>MEAVPRMPMIWLDLKEAGDFHFQPAVKKFVLKNYGENPEAYNEELKKLELLRQNAVRVPRDFEGCSVLRKYLGQLHYLQSRVPMGSGQEAAVPVTWTEIFSGKSVAHEDIKYEQACILYNLGALHSMLGAMDKRVSEEGMKVSCTHFQCAAGAFAYLREHFPQAYSVDMSRQILTLNVNLMLGQAQECLLEKSMLDNRKSFLVARISAQVVDYYKEACRALENPDTASLLGRIQKDWKKLVQMKIYYFAAVAHLHMGKQAEEQQKFGERVAYFQSALDKLNEAIKLAKGQPDTVQDALRFTMDVIGGKYNSAKKDNDFIYHEAVPALDTLQPVKGAPLVKPLPVNPTDPAVTGPDIFAKLV[2x];> KKKEEEDDDMKELENWAGSM

His domain protein tyrosine phosphatase (HD-PTP/PTPN23) is a tumor suppressor that regulates mitogenic receptor downregulation, endocytic recycling, and cell migration (Chen et al., 2012, Doyotte et al., 2008, Kharitidi et al., 2015, Lee et al., 2007, Ma et al., 2015, Manteghi et al., 2016). A central feature of HD-PTP function is the ability of its Bro1 domain to recruit CHMP4, the major subunit of the ESCRT-III membrane remodeling protein complex (Doyotte et al., 2008, Ichioka et al., 2007, Parkinson et al., 2015). Crystallographic structures of the HD-PTPBro1 domain in complex with the relevant binding regions of SARA, endofin, and all three human CHMP4 isoforms reveal that SARA and endofin binding is similar to that of CHMP4 at the conserved site, but critically extends into a neighboring specific pocket unique to HD-PTP. Altogether, this study identifies the Bro1 domain of HD-PTP as a highly selective interaction hub that coordinates recruitment of endosomal signaling adaptors versus MVB sorting and receptor degradation.

Y2H experiments confirmed that this region is also relevant for binding to HD-PTP, since CHMP4B lacking the C-terminal six amino acids (C4BΔCT) did not bind AlixBro1-V or HD-PTPBro1-CC, while full-length CHMP4B did. CoIP confirmed that CHMP4B-FL, but not C4BΔCT, binds to HD-PTPBro1-CC. Next, peptides designed from the C-terminal 18–20 residues of CHMP4A, CHMP4B, and CHMP4C were evaluated for binding to HD-PTPBro1. Interestingly, CHMP4 peptides showed much lower affinity to HD-PTPBro1 compared with the SARA/endofin peptides, with KD values of 132 ± 7 μM for CHMP4A, 85 ± 2 μM for CHMP4B, and 89 ± 1 μM for CHMP4C. For the CHMP4 peptides only 11 residues are clearly visible in the electron density maps, whereas 20 residues are visible for the SARA and endofin peptides. All three CHMP4 peptides bind in the same way across helices H5, H6, and H7 of HD-PTPBro1, and form similar van der Waals contacts with a number of conserved residues, including the critical L202/I206 pair. Additional contacts occur with hydrophobic residues at the proline-rich C-terminal region of HD-PTPBro1 (see Table 2 for a list of all interactions). The main CHMP4 anchoring residues are a Leu and a Trp present in all three isoforms (L217 and W220 in CHMP4A and CHMP4B, L228/W231 in CHMP4C), which contact HD-PTPBro1 residues L189, L202, and I206 from two hydrophobic pockets between H5 and H6 and H6 and H7. Thus, binding of CHMP4A/B/C to HD-PTPBro1 requires rearrangement of these side chains to accommodate the critical CHMP4 Leu and Trp residues. Binding of full-length CHMP4B to HD-PTPBro1-CC was unaffected by the T145K mutation, confirming that access to the S site is not required for CHMP4 binding but is critical for interaction with endofin and presumably SARA as well.>GAMENPLKRLLVPGEEWEFEVTAFYRGRQVFQQTISCPEGLRLVGSEVGDRTLPGWPVTLPDPGMSLTDRGVMSYVRHVLSCLGGGLALWRAGQWLWAQRLGHCHTYWAVSEELLPNSGHGPDGEVPKDKEGGVFDLGPFI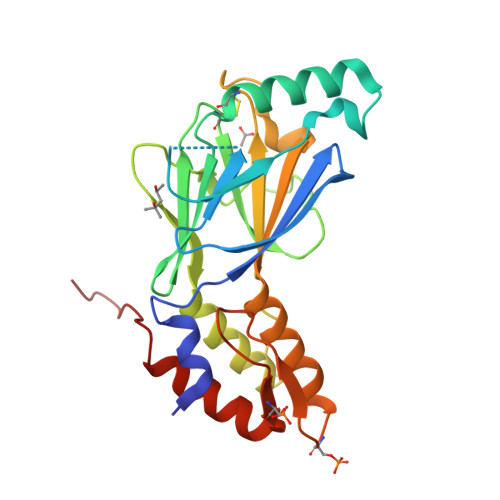VDLITFTEGSGRSPRYALWFCVGESWPQDQPWTKRLVMVKVVPTCLRALVEMARVGGASSLENTVDLHISNSHPLSLTSDQYKAYLQDLVEGMDFQGPGES[4x]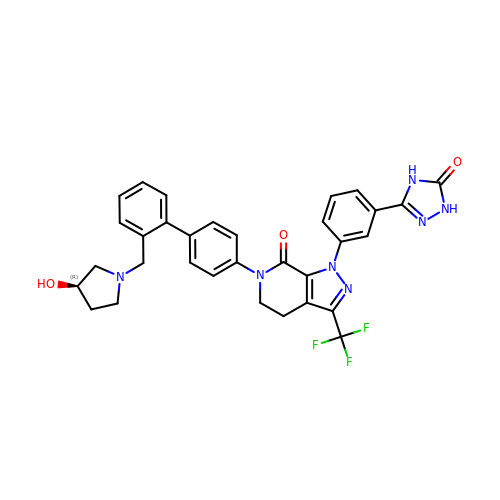(R)-6-(2'-((3-hydroxypyrrolidin-1-yl)methyl)biphenyl-4-yl)-1-(3-(5-oxo-4,5-dihydro-1h-1,2,4-triazol-3-yl)phenyl)-3-(trifluoromethyl)-5,6-dihydro-1h-pyrazolo[3,4-c]pyridin-7(4h)-one | C32 H28 F3 N7 O3 | YBWAYLVOTDFQQI-XMMPIXPASA-N> M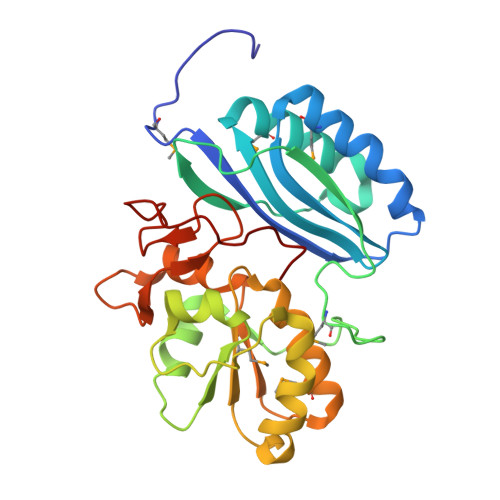GHHHHHHSHMVKDIIIASFYKFIPLNDFRSLREPILTKMHEIGIKGTIILAHEGVNGGFAGNREQMNVFYDYLRSDSRFADLHFKETYDNKNPFDKAKVKLRKEIVTMGVQKVDPSYNAGTYLSPEEWHQFIQDPNVILLDTRNDYEYELGTFKNAINPDIENFREFPDYVQRNLIDKKDKKIAMFCTGGIRCEKTTAYMKELGFEHVYQLHDGILNYLESIPESESLWEGKCFVFDDRVAVDQKLDRVYPQLPQDYKYEREQK>PSGAKLLQILNVRVVGSGERVVVLSHGFGTDQSAWSRVLPYLTRDHRVVLYDLVCAGSVNPDHFDFRRYDNLDAYVDDLLAILDALRIPRCAFVGHSVSAMIGILASIRRPDLFAKLVLIGASPRFLNDSDYHGGFELEEIQQVFDAMGANYSAW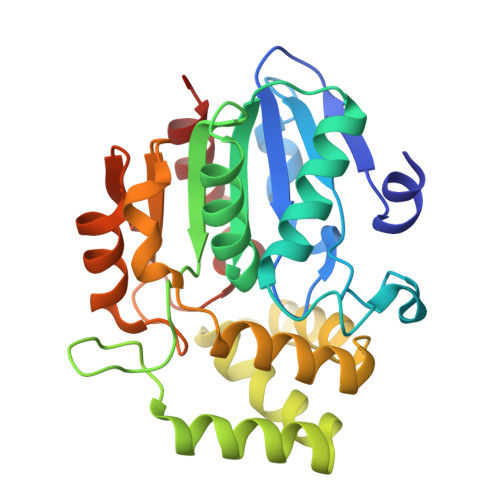ATGYAPLAVGADVPAAVQEFSRTLFNMRPDISLHVCQTVFKTDLRGVLGMVRAPCVVVQTTRDVSVPASVAAYLKAHLGGRTTVEFLQTEGHLPHLSAPSLLAQVLRRALARY[2x]> MSVPVQHPMYIDGQFVTWRGDAWIDVVNPATEAVISRIPDGQAEDARKAIDAAERAQPEWEALPAIERASWLRKISAGIRERASEISALIVEEGGKIQQLAEVEVAFTADYIDYMAEWARRYEGEIIQSDRPGENILLFKRALGVTTGILPWNFPFFLIARKMAPALLTGNTIVIKPSEFTPNNAIAFAKIVDEIGLPRGVFNLVLGRGETVGQELAGNPKVAMVSMTGSVSAGEKIMATAAKNITKVCLELGGKAPAIVMDDADLELAVKAIVDSRVINSGQVCNCAERVYVQKGIYDQFVNRLGEAMQAVQFGNPAERNDIAMGPLINAAALERVEQKVARAVEEGARVAFGGKAVEGKGYYYPPTLLLDVRQEMSIMHEETFGPVLPVVAFDTLEDAISMANDSDYGLTSSIYTQNLNVAMKAIKGLKFGETYINRENFEAMQGFHAGWRKS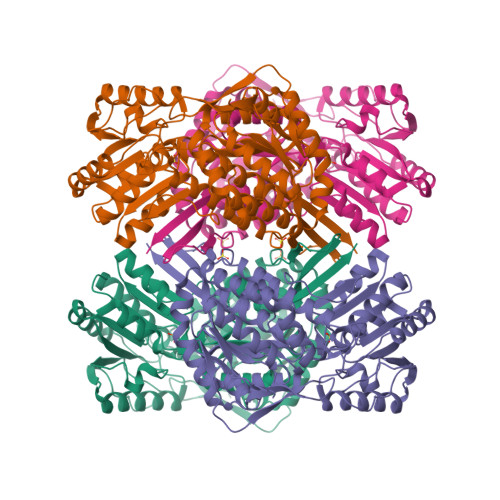GIGGADGKHGLHEYLQTQVVYLQS> PVLNLNDPQAVERYEEFMRQSPYGQVTQDLGWAKVKNNWEPVDVYLEDDQGAIIAAMSMLLGDTPTDKKFAYASKGPVMDVTDVDLLDRLVDEAVKALDGRAYVLRFDPEVAYSDEFNTTLQDHGYVTRNRNVADAGMHATIQPRLNMVLDLTKF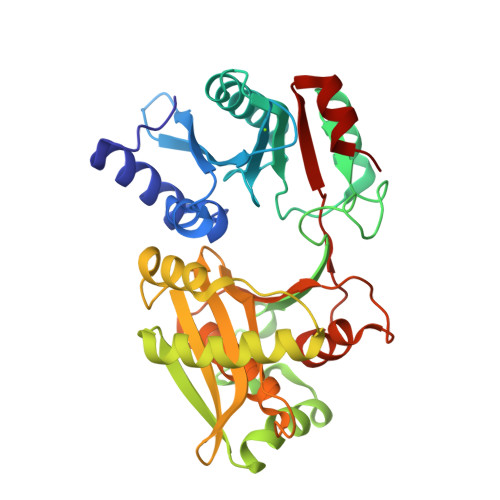PDAKTTLDLYPSKTKSKIKRPFRDGVEVHSGNSATELDEFFKTYTTMAERHGITHRPIEYFQRMQAAFDADTMRIFVAEREGKLLSTGIALKYGRKIWFMYAGSMDGNTYYAPYAVQSEMIQWALDTNTDLYDLGGIESESTDDSLYVFKHVFVKDAPREYIGEIDKVLDPEVYAELVKD>GAMGSHPMCKEHEDEKINIYCLTCEVPTCSMCKVFGIHKACEVAPLQ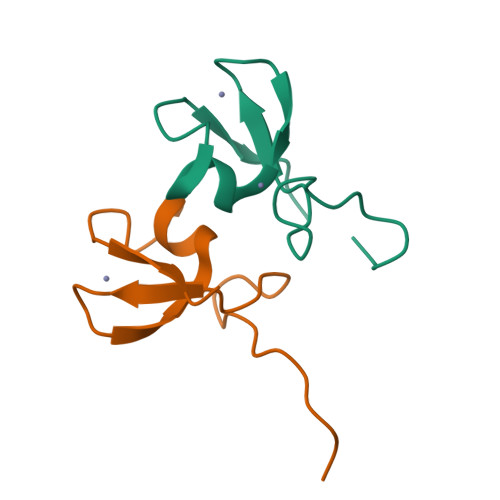S[3x]>GMKVTFLGHAVVLIEGKKNIIIDPFISGNPVCPVKLEGLPKIDYILVTAGHGDHLGDAVEIAKKNDATVISNYEICHYLGKKGVKTHAMHIGGSYLFDFGRVKMTPAVHGSGILDGDSMIYGGNPSGFLITIEGKKIYHAGDTGLTREM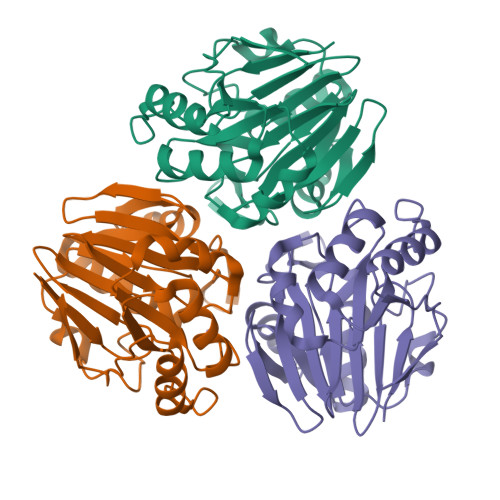ELLAEENVDVAFLPIGGNFVMDVEDAVRAAVMIKPKKVVPMHYGTWELIFADVELFKKKVEEKGVECVILEPGESLEL[3x]> MVFKKV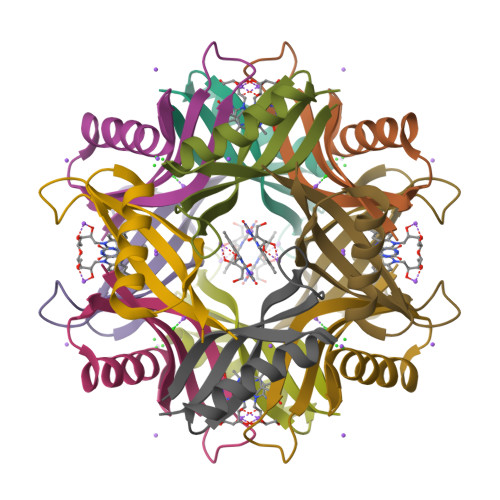LLTGTSEESFTAAADDAIDRAEDTLDNVVWAEVVDQGVAIGAVEERTYQTEVQVAFELD> MSDVLIRDIPDDVLASLDAIAARLGLSRTEYIRRRLAQDAQTARVTVTAADLRRLRGAVAGLG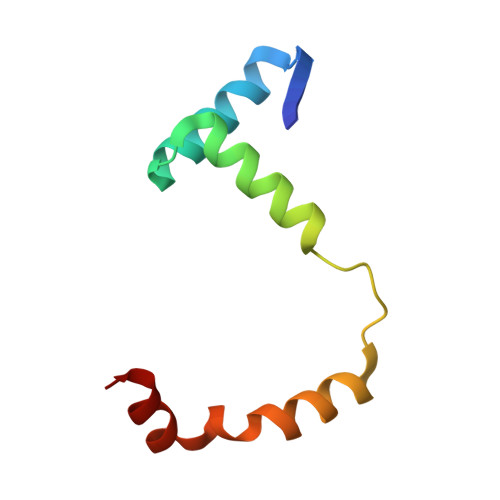DPELMRQAWR> MGEQVVKPTDERIIDPSTANTQLTGGVCYNTTSGGNKPLAGSPYGYEFWIDTGGGVCSFCWYGADQGGGAAFKATWTNPHDFLGRLGYFWNENKPYSHYENIYCGFNYTRSGRKTAGDYSYIGIYGWSRNPSASNSNERLIEYYIVEDWFGNQWQADTSPMGINTTGGTVMGSFTVDGSSYQIIKNTRVNQPSIEGDKTFVQYFSIRQSPRKSGTISITEHFKKWEKLGMKLGDNMYECKFLIEAGAGEG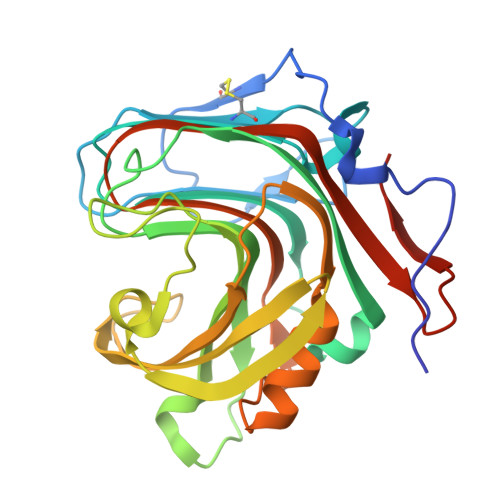FFDARLIQFYRADNEGNILQITPLEHHHHHH>[4x]GMRVDKHEVRVGELAAGQPLSLPVYRFKGKGAGPSVYIQAN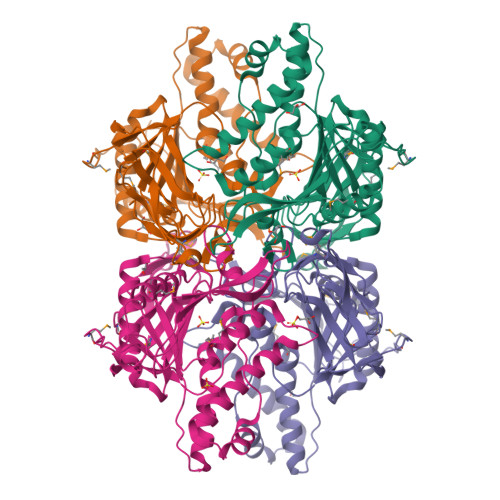VHGAEVQGNAVIYQLMKLLEHYELLGDISLVPLANPLGINQKSGEFTLGRFDPITGVNWNREYLDHGFNIEVWYQEHSHLDDDTLITAFRATLVEECARRLNNPWGVTTGHRLAVTLQSMAHRADIVLDLHTGPKSCKHLYCPEYERSAAQYFSIPYTLLIPNSFGGAMDEAAFVPWWTLAEVASSHGRELGVRVSALTLELGSQERIDLDDALEDAEGILAYLSHRGVIAETVLPKPMKRYGCFLKNYRKFHAPKAGMVEYLGKVGVPMKATDPLVNLLRLDLYGTGEELTVLRLPEDGVPILHFASASVHQGTELYKVMTKVFEL MATs are an essential and ubiquitous enzyme family found in all domains of life. 38 MATs catalyze the condensation of ATP with methionine to generate S‐adenosylmethionine (SAM)—an essential molecule involved in numerous biological processes, including RNA, DNA, protein and small molecule methylation, polyamine synthesis, and production of enzyme cofactors. 39 Analysis of available crystal structures reveals that bacterial MATs are predominantly dihedral homotetramers (D2 symmetry group), that is, comprised of dimers of dimers 40. Two deep cavities harboring active sites are located directly in this dimeric interface, making the homodimer the obligatory functional unit.

Further, whereas the small interface of NgMAT has no salt‐bridges, the small interface of EcMAT contains eight: Lys98 in each EcMAT subunit forms a salt‐bridge network with Asp64 and Glu67 of the opposing subunit. 26 To explore this hypothesis, we generated two reciprocal mutants, swapping the salt‐bridge‐forming residues in the EcMAT small interface (Lys98 and Glu67) with those of NgMAT (Gln98 and Lys67), and vice versa. Additionally, we solved the crystal structure EcMATmut at 1.6 Å resolution and found that the protein assembles into a homotetramer that is highly structurally similar to EcMAT. PISA analysis of the small EcMATmut interface revealed that its hydrophobicity (ΔG i /area) increased by approximately 30% compared to that of EcMAT (11.8 vs. 9.0 cal/mol/Å2, respectively), whereas the net per‐residue electrostatic contribution (ΔΔG elec) of EcMATmut was comparable to that of NgMAT. Following purification of the E. coli mutant (EcMATmut) and the N. gonorrhoeae mutant proteins, we determined that the removal of the salt‐bridges did not affect the catalytic activity of EcMATmut, while the addition of salt‐bridge‐forming residues to NgMAT resulted in substantial aggregation. Removal of the salt‐bridges did not change the kinetic stability of the tetrameric complex. Strikingly, while at equilibrium the tetrameric fraction of EcMAT constituted 30%, the tetrameric fraction of EcMATmut was only 5%. Based on these measurements we calculated the tetramer‐dimer equilibrium dissociation constant, K d (see Section 4) and determined that the K d of EcMAT was approximately 11‐fold lower than that of EcMATmut (8.2 vs. 90.3 μM, respectively). Interestingly, removal of glycerol from the incubation buffer resulted in a dramatic and increasing aggregation of the dimeric fraction of EcMATmut, which, led to a loss of over 90% of the tetrameric fraction after 120 hr of incubation. We found that the rate of SAM accumulation by EcMATmut is approximately 60% lower than that of EcMAT.

> MAKHLFTSESVSEGHPDKIADQISDAVLDAILEQDPKARVACETYVKTGMVLVGGEITTSAWVDIEKITRNTVREIGYVHSDMGFDANSCAVLSAIGQQSPDINQGVDRADPLEQGAGDQGLMFGYATNETDVLMPAPITYAHRLVQRQAEVRKNGTLPWLRPDAKSQVTFQYDDGKIVGIDAVVLSTQHSEEIDQKSLQEAVMEEIIKPILPAEWLTSATKFFINPTGRFVIGGPMGDCGLTGRKIIVDTYGGMARHGGGAFSGKDPSKVDRSAAYAARYVAKNIVAAGLADRCEIQVSYAIGVAEPTSIMVETFGTEKVPSEQLTLLVREFFDLRPYGLIQMLDLLHPIYKETAAYGHFGREHFPWEKTDKAQLLRDAAGLKHHHHHH>MNITIYDVAREANVSMATVSRVVNGNPNVKPTTRKKVLEAIERLGYRPNAVARGLASKKTTTVGVIIPDISSIFYSELARGIEDIATMYKYNIILSNSDQNMEKELHLLNTMLGKQVDGIVFMGGNITDEHVAEFKRSPVPIVLAASVEEQEETPSVAIDYEQAIYDAVKLLVDKGHTDIAFVSGPMAEPINRSKKLQGYKRALEEANLPFNEQFVAEGDYTYDSGLEALQHLMSLDKKPTAILSATDEMALGIIHAAQDQGLSIPEDLDIIGFDNTRLSLMVRPQ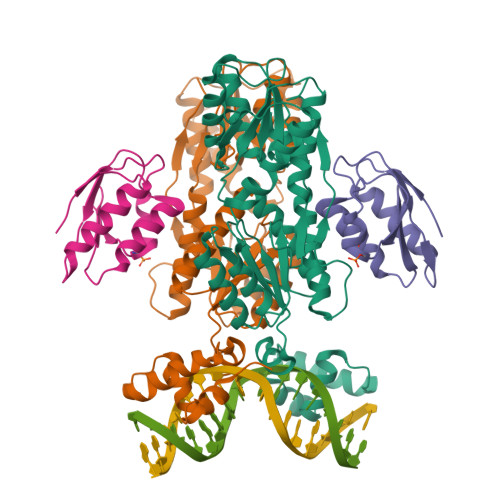LSTVVQPTYDIGAVAMRLLTKLMNKEPVEEHIVELPHRIELRKSTKSHHHHHH[2x];>AQKTFKVTADSGIHARPATVLVQTASKYDADVNLEYNGKTVNLKSIMGVMSLGIAKGAEITISASGADENDALNALEETMKSEGLGE[2x]Rab8a is one of several Rab GTPases that are substrates of leucine-rich repeat kinase 2 (LRRK2), a serine/threonine kinase that is linked to Parkinson's disease. Rab8a is phosphorylated at T72 (pT72) in its switch 2 helix and recruits the phospho-specific effector RILPL2, which subsequently regulates ciliogenesis. Rabs comprise the largest group (∼70 members) of the Ras superfamily, and they cycle between an active GTP bound and inactive GDP form to regulate membrane trafficking in eukaryotic cells. LRRK2 phosphorylation of Rab8a and Rab10 also promoted interaction with two poorly studied scaffolding proteins termed RILPL1 (Rab interacting lysosomal protein-like 1) and RILPL2 (Steger et al., 2017), that were previously implicated in regulating ciliogenesis.

Here, we describe the crystal structure of T72 phosphorylated Rab8a(GTP) in complex with a minimal phospho-Rab binding domain of RILPL2 at 1.8 Å resolution. For these studies we utilized a mutant of the globular G-domain of Rab8a (Q67L, residues 1–181) that binds GTP constitutively. Full-length RILPL2 complexes failed to crystallize, but the phospho-Rab binding domain of RILPL2 (residues 129–165) yielded crystals in complex with pRab8a. The complex of pRab8a(GTP):RILPL2 is organized as a heterotetramer in the asymmetric unit, with a central parallel α-helical dimer of the phospho-Rab binding domain of RILPL2 bridging two molecules of pRab8a via hydrophobic and polar interactions. Each pRab8a molecule interacts with both α helices of the effector, burying approximately 625 Å2 of surface area at each interface. The N termini of the RILPL2 dimer (N129RL2-T134RL2) cross over in an extended conformation preceding the first α-helical turn, forming an X-shaped cap (X-cap) over the coiled coil. The X-cap facilitates interactions of both monomers of RILPL2 with a single phosphorylated switch 2 of pRab8a. The phosphate moiety from pT72 interacts with the guanidino group (NH1/NH2) of R132RL2 on both sides of the symmetric complex, with O/N distances between 2.5 and 2.9 Å. In addition to electrostatic contacts, the X-cap residue F133RL2 contributes to a complementary hydrophobic interface with F70R8 and I73R8 from switch 2. Mutation of K149RL2—which forms a salt bridge with D44R8 (switch 1)—also abolishes the interaction between RILPL2 and pRab8a.

>GSHMAKTYDYLFKLLLIGDSGVGKTCVLFRFSEDAFNSTFISTIGIDFKIRTIELDGKRIKLQIWDTAGLERFRTITTAYYRGAMGIMLVYDITNEKSFDNIRNWIRNIEEHASADVEKMILGNKCDVNDKRQVSKERGEKLALDYGIKFMETSAKANINVENAFFTLARDIKAKMDKKLEGNS[2x];>[2x]HHHHHHNRPRFTLQELRDVLQERNKLKSQLLVVQEELQCYKSG> QVKPFSFVRDTDPVQLVNFLQSEHPQTI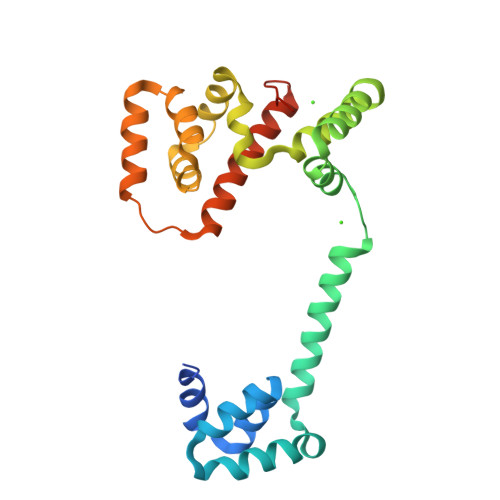AVVLSYLDPPVAAQILGALPEELQTEVLKRIALLERTSPEVVKEIERNLEKKISGFVSRTFSKVGGIDTAAEIMNNLDRTTEKKIMDKLVQENPELADEIRRRMFVFEDILKLDDRSIQLVLREVDTRDLALALKGASDELKEKIFKNMSKRAAALLKDELEYMGPVRLKDVEEAQQKIINIIRRLEEAGEIVIARGGGEELIM>[2x]MAHHHHHHHHHANVVVCIKQVPDTTNVRIDRKTNNLVREGVPSIINPDDERALELASQLKEKFGATVYVITMGPPQAKEALKDAIAFGLDEAVHLSDRTFAGADTLATTYTLYWGIKKIEERIGKIDLILTGKQAVDGDTGQVGPGLATRFGYALGAYVVRIEEIDPEKKEMVIVRRLDQGFEKIRLKLPAVLTITDELNKPRYADLPNLIRAIRYEPIVWTHKDLGLDPKKCGFFGSPT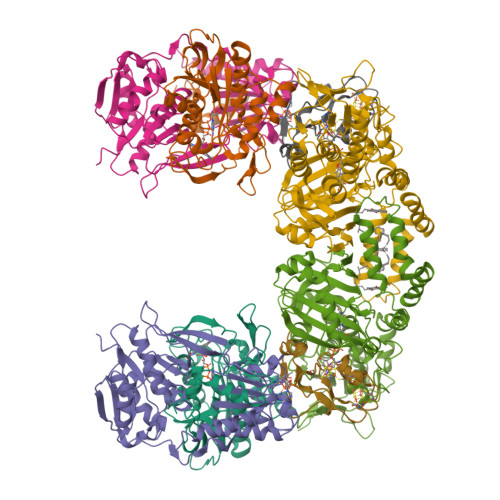RVVSTNIPPARKGGDIISKNEDPEVAAEKLIEALKKFEAVRLVEALKPVLEGEKDE;>[2x]MSEKKIIFVLIEHHGGKAHPVSWELIGKARDLASKLENSEVWGVLLGEGLESVAKEAIQRGADKVLYVKNREFNTYVNYLYKKALVDMVRKYRPEIFLIGATLEGRELAGMVATELETGLTADCTGLDIIPDKKLLAMTRPTFGGNLMATIMCPDHRPQMATVRPGVMKELPPDPERTGEIIEEEYDLGTFDKLIEILETIPLQTQVNLEYAPVVVAGGKGVGGPEGFKKLKELADLLGGEVGASRAAVKAGWISPEHQVGQTGKTVRPVLYFACGISGAIQHVVGIKESEIIVAINIDEKAPIFDIADIGIVGDLHKVVPALTAKLRELLNKSGVKK;>[2x]MKIEFDVVVVGAGPSGLSCAYVLAKNGLKVAVVEKGEYPGSKNVMGGVLYVHPLKEIMPDFLEKAANSKALERNVIEQNLWLLGNEGVIKIGHRNVEWKENPNAFTVLRANFDRWFAQEVEKAGALIIPKTKVEDFLRNEKGEIAGVVTSRPKGEIHSKAVVIAEGVNPILTMKAGLRKEDLKPHMVAVAVKEVISVPEDVVNRVFGVEGNDGATIELLGSWSEGMFGMGFLYANRSSVSLGCGVLLEDLRKKKIKPYQLLENLKNHPVISDMLGEYRNNTMEYLAHLIPEGGYYAMPKVYGDRVLVCGDAAMLVNSIHREGSNHAITSGRLAAETLLEAFEKGDFSEKILKNYYLRLKESFILKDLEKYKDLMPTMEKNHQFVEIYPDLANDALKRFLQVDGTPKWDVQKQIADMVLSRRSLIGISLDLLRFWRAVR;>[2x]MRIEDKLYLNRYRTDEENPHLKIKDESICAEKCSDRPCVSCCPADVYEWTESGMEVKFEGCLECGTCRIVCPFGNIEWNYPRGNYGVLYKFG> LDGPYQPTTFTPPIDYWILINSNTNGVVYESTNNSDFWTA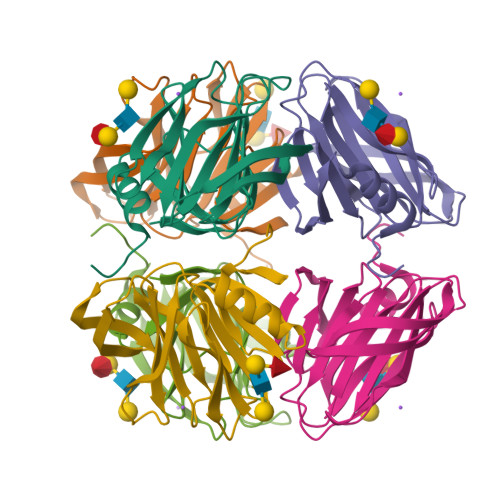VVAIEPHVNPVDRQYTVFGENKQFNVRNDSDKWKFLEMFRSSSQNEFYNRRTLTSDTKLVGILKYGGRIWTFHGETPRATTDSSNTANLNDISIIIHSEFYIIPRSQESKCNEYINNGLLEHH>[3x]SNAMKQIIDIENWERKENFNFFRHFQNPQLSITSEVECGGARQRAKAAGQSFFLHYLY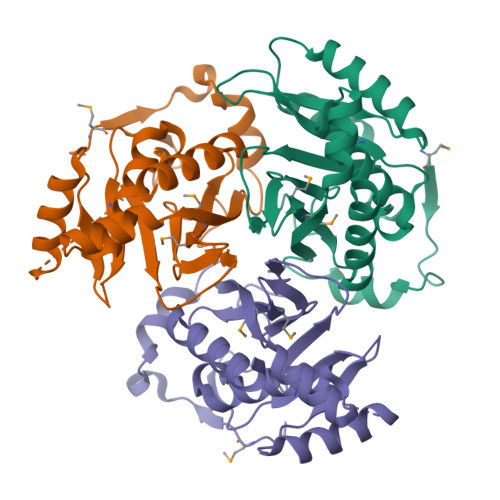AVLRAANEIPEFRYRIDPDGRVVLYDTIDMLSPIKIKENGKFFTTRFPYHNDFDTFYQEARLIIDAIPEDGDPYAAENEEVADGDYGLILLSATPDLYFTSITGTQEKRSGNNYPLLNAGKAIIREGRLVMPIAMTIHHGFIDGHHLSLFYKKVEDFLK> SNPKFENIAEGLRALLARSHVERTTDEGTWVAGVFVYGGSKTSLYNLRRGTALA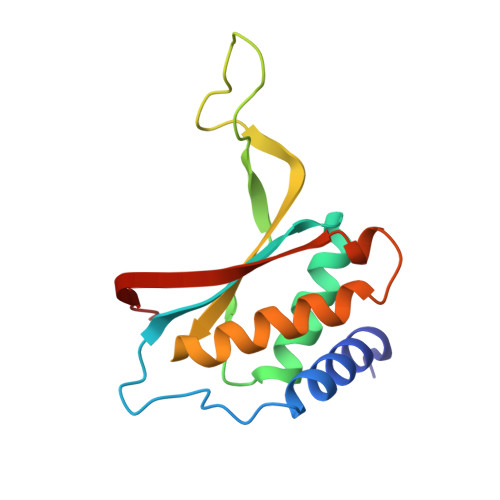IPQCRLTPLSRLPFGMAPGPGPQPGPLRESIVCYFMVFLQTHIFAEVLKDAIKDLVMTKPAPTCNIRVTVCSFDDGVDLP>GSEFELMTHSVSPIGYIRSCFMEKFAIPRQPLLAPAARGTLELLPPFDQVEALEGLEQVSHVWLLFLFHQALEDKPRLKVRPPRLGGNRSLGVFATRATHRPNGIGQSVVRLEGFEAGRLWLSGIDLLDGTPVLDIKPYVPYADA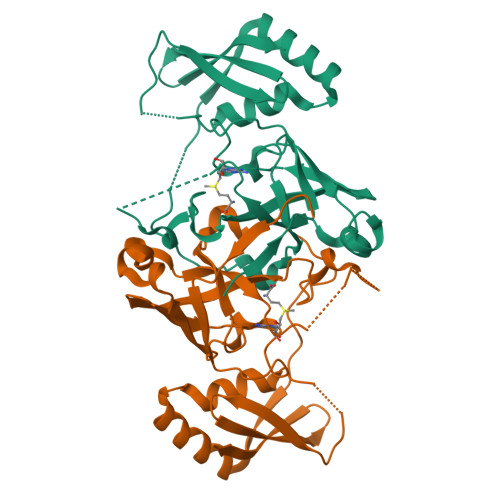VADARNGIADAPPPGIAVEWSEQARRQAHEHGQRLRQPVAELIEQCLAQDPRPAYQKPEPGRRYGVRLWDLDVHWHYPRPDLIRVLDVAGGD[2x]> MLAKRIIACLDVKDGRVVKGSNAENLRDSGDPVELGKFYSEIGIDELVFLDITASVEKRKTMLELVEKVAEQIDIPFTVGGGIHDFETASELILRGADKVSINTAAVENPSLITQIAQTFGSQAVVVAIDAKRVDGEFMVFTYSGKKNTGILLRDWVVEVEKRGAGEILLTSIDRDGTKSGYDTEMIRFVRPLTTLPIIASGGAGKMEHFLEAFLAGADAALAASVFHFREIDVRELKEYLKKHGVNVRLEGL

We have studied this problem on the example of the mobile active site β1α1-loop (loop1) of the (βα)8-barrel enzyme HisF, which is the cyclase subunit of imidazole glycerol phosphate synthase. Prokaryotic ImGPS enzymes (including the ImGPS from T. maritima) form heterodimeric bienzyme complexes that consist of the cyclase HisF and the glutaminase HisH subunit, which supplies ammonia by glutamine hydrolysis. The active site of HisF is located at the C-terminal face of the central β-barrel, where two conserved aspartate residues, D11 and D130, catalyze the cyclase reaction. Based on the conformation of the loop that connects strand β1 with helix α1 (loop1), these structures can be separated into an open conformation, where loop1 is flipped toward the outer α-helical barrel ring, a detached conformation, where loop1 is not visible in the electron density and presumably flexible and a closed conformation, where loop1 closes over the active site.

To assess whether the mutations have an influence on the conformation of loop1 we determined the structures of the HisF-G20P and HisF-F23A variants by X-ray crystallography. In summary, our crystallography, proteolysis, NMR, and simulation data demonstrate that the HisF-G20P and HisF-F23A variants have opposing effects on the conformation of loop1. However, whereas loop1 primarily samples the open conformation in the HisF-G20P variant, the loop1 population shifts toward the highly flexible detached conformation in the HisF-F23A variant. Whereas the G20P and F23A substitutions decrease the kcat of wt-HisF by several orders of magnitude, the F38A substitution has no effect on the steady-state catalytic parameters. Instead, the G20P and F23A substitutions likely influence turnover via alterations in the closed conformation of loop1. In contrast, in the case of loop1 variants HisF-F23A and HisF-G20P, kobs, increased linearly with increasing concentrations of PrFAR, which is indicative of a simple binding process without involvement of conformational changes. The HisF-G20P and HisF-F23A variants on the other hand interact with the substrate via a one step binding mechanism as loop1 is, in those cases, unable to close properly over the substrate.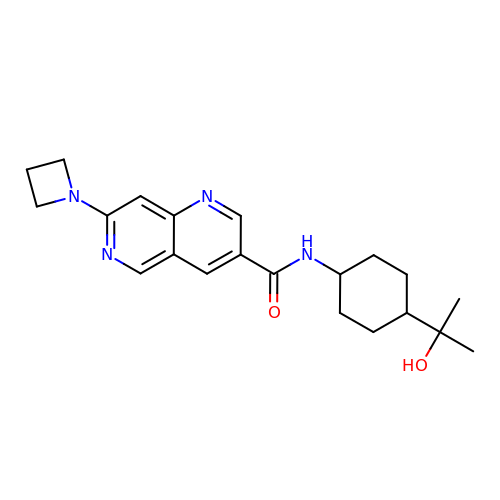7-(azetidin-1-yl)-~{N}-[4-(2-oxidanylpropan-2-yl)cyclohexyl]-1,6-naphthyridine-3-carboxamide | C21 H28 N4 O2 | YBOJDFGHCNHNOW-QAQDUYKDSA-N>MNINIVTIGKLKEKYLKQGIEEYTKRLSAYAKIDIIELPDEKAPENLSDQDMKIIKDKEGDRILSKI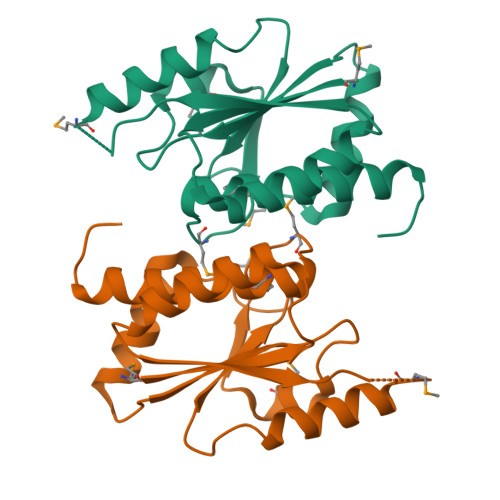SPDAHVIALAIEGKMKTSEELADTIDKLATYGKSKVTFVIGGSLGLSDTVMKRADEKLSFSKMTFPHQLMRLILVEQIYRAFRINRGEPYHKLEHHHHHH[8x]trans-4-{4-[7-amino-2-(1,2,3-benzothiadiazol-7-yl)-3-chlorofuro[2,3-c]pyridin-4-yl]-1H-pyrazol-1-yl}cyclohexanol 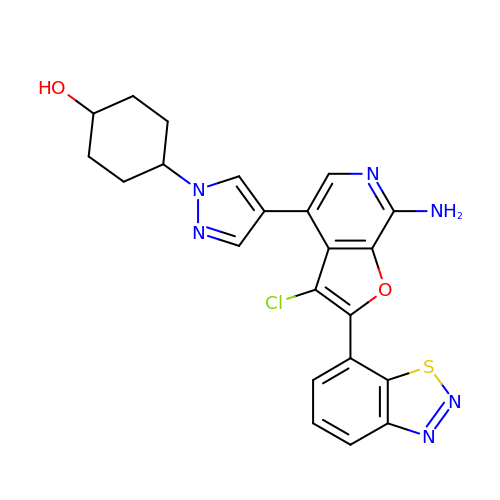| C22 H19 Cl N6 O2 S | IXXBWYJJOYSCNJ-JOCQHMNTSA-N~{N}-[4-(1-methylpiperidin-4-yl)phenyl]-7-(1-methylpyrazol-4-yl)quinazolin-2-amine 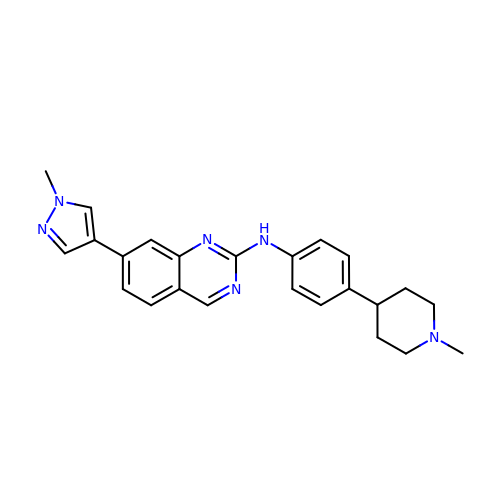| C24 H26 N6 | VCCYOHCOICDUFL-UHFFFAOYSA-N> MSKDIKQVIEIAKKHNLFLKEETIQFNESGLDFQAVFAQDNNGIDWVLRLPRREDVMPRTKVEKQALDLVNKYAISFQAPNWIIYTEELIAMKKLDGVPAGTIDHNIGNYIWEIDINNVPELFHKSLGRVLAELHSIPSNKAAALDLVVHTPEEARMSMKQRMDAVRAKFGVGENLWNRWQAWLNDDDMWPKKTGL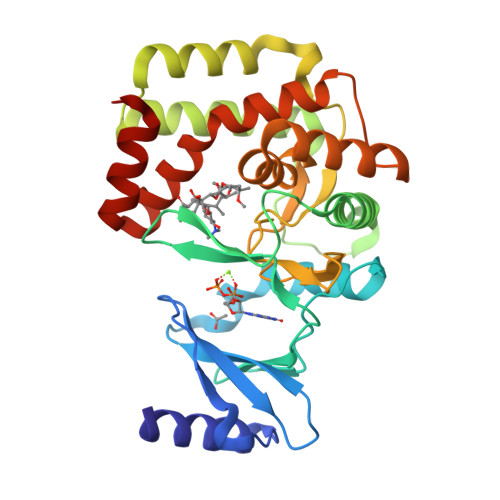IHGDVHAGHTMIDKDANVTGLIDWTEAKVTDVSHDFIFNYRAFGEEGLEALILAYKEIGGYYWPKMKEHIIELNAAYPVSIAEFALVSGIEEYEQMAKEALEVQGS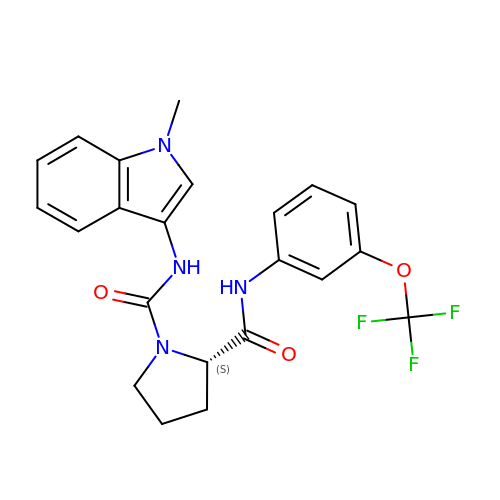(2~{S})-~{N}1-(1-methylindol-3-yl)-~{N}2-[3-(trifluoromethyloxy)phenyl]pyrrolidine-1,2-dicarboxamide | C22 H21 F3 N4 O3 | IRTQBCRDCGFMII-IBGZPJMESA-N> SVLQVLHIPDERLRKVAKPVEEVNAEIQRIVDDMFETMYAEEGIGLAATQVDIHQRIIVIDVSENRDERLVLINPELLEKSGETGIEEGCLSIPEQ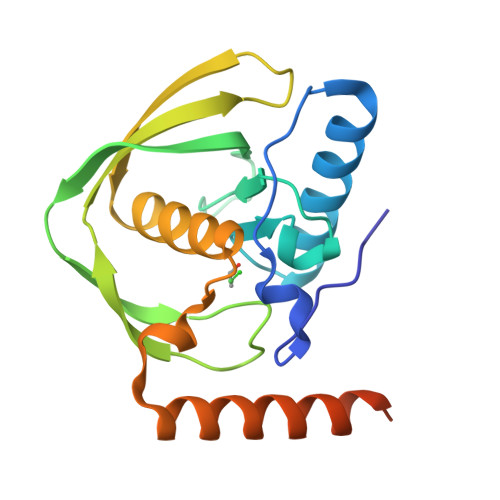RALVPRAEKVKIRALDRDGKPFELEADGLLAICIQHEMDHLVGKLFMDYLSPLKQQRIRQKVEKLDRLKARAPNSSSVDKLAAALEHHHHHH>[4x]SKPQPIAAANWKCN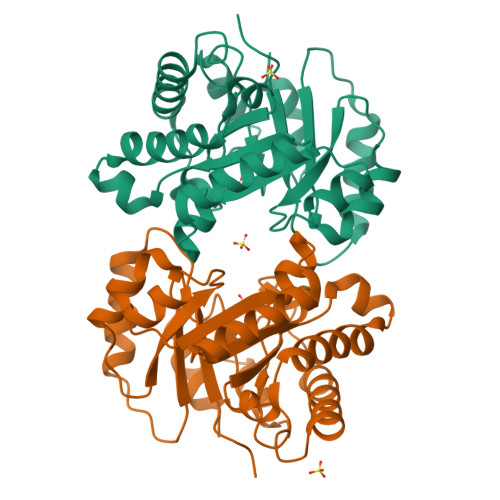GSQQSLSELIDLFNSTSINHDVQCVVAPSFVHLAMTKERLSHPKFVIAAQNAGNADGLASLKDFGVNWIVLGHSERRAYYGETNEIVADKVAAAVASGFMVIACIGETLQERESGRTAVVVLTQIAAIAKKLKKADWAKVVIAYEPVWAIGTGKVATPQQAQETHALIRSWVSSKIGADVAGELRILYGGSVNGKNARTLYQQRDVNGFLVGGASLKPEFVDIIKATQ> KKAIVRLSIPMMIGMSVQTLYNLADGIWVSGLGPESLAAVGLFFPVFMGIIALAAGLGVGTSSAIARRIGARDKEGADNVAVHSLILSLILGVTITITMLP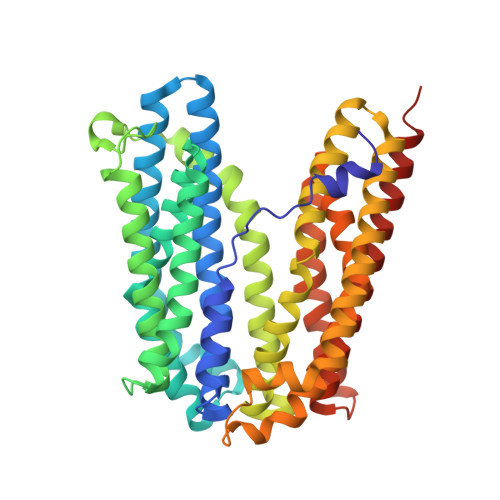AIDSLFRSMGAKGEAVELAIEYARVLLAGAFIIVFNNVGNGILRGEGDANRAMLAMVLGSGLNIVLDPIFIYTLGFGVVGAAYATLLSMVVTSLFIAYWLFVKRDTYVDITLRDFSPSREILKDILRVGLPSSLSQLSMSIAMFFLNSVAITAGGENGVAVFTSAWRITMLGIVPILGMAAATTSVTGAAYGERNVEKLETAYLYAIKIAFMIELAVVAFIMLFAPQVAYLFTYSESAQVIKGDLISALRTLPVFLVLTPFGMMTSAMFQGIGEGEKSLILTIFRTLVMQVGFAYIFVHYTTLGLRGVWIGIVIGNMVAAIVGFLWGRMRISALKKTSA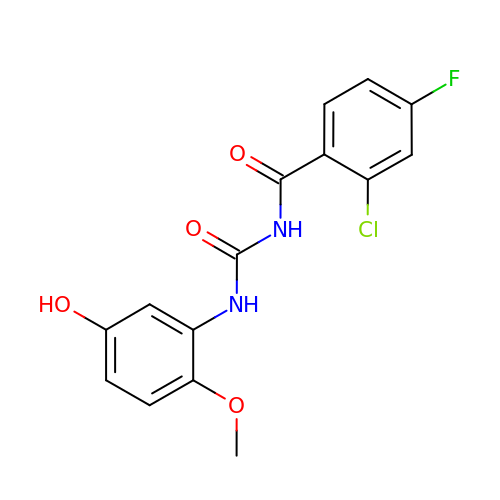N-(2-CHLORO-4-FLUOROBENZOYL)-N'-(5-HYDROXY-2-METHOXYPHENYL)UREA | C15 H12 Cl F N2 O4 | RFOBTYLRURSVJE-UHFFFAOYSA-N However, we were successful in performing structural study of a newly discovered bacterial RNA repair complex consisting of three proteins named Pnkp1, Rnl and Hen1, which form a heterohexamer in vitro. Since the newly found RNA repair system possesses elements of both T4 and Pnkp–Hen1 RNA repair systems, it can be regarded as a hybrid RNA repair system. Therefore, the Pnkp1–Rnl–Hen1 heterohexamer is likely the functional unit of a new bacterial RNA repair system in vivo. Because the Pnkp1–Rnl–Hen1 RNA heterohexamer possesses two identical copies of each enzymatic activity, a total of eight active sites are present in the complex, same as in the RNA repair complex of the Pnkp–Hen1 heterotetramer.

To provide insight into the mechanism of RNA repair by the Pnkp1–Rnl–Hen1 heterohexamer, we soaked crystals with adenosine triphosphate (ATP) before data collection, which resulted in a crystal structure with cofactors occupying all active sites. Guided by the locations of these cofactors, and aided by the published structural homologues of Pnkp1 and Hen1 in complex with nucleic acids as well as the model of RNA in complex with the ligase module of Pnkp–Hen1, we manually docked short single-stranded RNAs into the four active sites located in the inner rim of one ring structure. The docking model shows that, while the reacting ends of single-stranded RNAs (not observed in Fig. 6a) are placed in the active site, the opposite ends point to a vacant space at the centre of the ring structure, indicating that a RNA substrate approaches each repair unit from this vacant space for RNA repair. The 5′ end of the damaged RNA would first enter the kinase site for phosphorylation and, at the same time, the 3′-end of the damaged RNA would go into the phosphatase site for dephosphorylation. Because of highly efficient 5′-phosphorylation carried out by the kinase domain of Pnkp1, the 5′ end would be the first to enter the ligase site, where it could be activated with 5′-adenylation by RNA ligase. On the other hand, after 3′-dephosphorylation carried out by the phosphatase domain of Pnkp1, the 3′ end could make a detour to the methyltransferase site of Hen1 for 2′-O-methylation before joining the 5′ end in the ligase site. With the presence of both processed ends in the ligase site, RNA ligation occurs, which results in repaired RNA with 2′-O-methylation. Among the four active sites located on the inner rim of the same ring structure, the kinase and phosphatase active sites are from one unit of the Pnkp1–Rnl–Hen1 heterotrimer, and the methyltransferase and ligase active sites are contributed from the other unit. Our structure revealed that the methyltransferase site is located between the phosphatase and ligase sites, providing the 3′ end of the damaged RNA maximal opportunity to be 2′-O-methylated after dephosphorylation but before ligation.

>MSAKNNTHHFPKLLILVGAPGSGKSTFARYFIRTEDNWVRVNRDDFRLMQFGDSLMSPFYEERITKMVEASVIALLKNRTNVIIDATNSSLRSLQDMVHTYTEYADISFKVFDLPVEELVKRCDKRCEQTGKFIPKSAIEKHVTQLQYTKEKFDFKPIPRALKETSLTYADQDTSLPKAVICDLDGTLSLLNGRDPYNASTADQDLLNTPVAMVLKMAKQQGYKVILLSGRENAYREPTERFLAKYQIDYDLLLMRDTNDYRKDNIIKKELFLEEIQGKYFVEFLLDDRNQVVDMWRRELALPCFQVNYGDF[2x];>[2x]MEDKTLIKKRIDWFCKNKINAFSPTISPAPKSVERNEIESLYEGILWFVLNGVKEIVIEKKYMGSYCDIYLHRRLEDTYLVSRNGYKINHLDQEQCLRALQGLHDRFSWDGVELRIIQSELMPWSILGKGLINNEFSAYYISHEIHAEYLVQSSLYEKLQKIQQEPAYLSFVADAKVLSAKELKDKYPMHIIRQYQSIRDFKFLDLPHYQQNIQLFKRQLDIFGKEAAPFFKPFNILKEVYTDGREHFVNDNLSFQQINDDDFLHYQFTDREDFEAKYPQIRAWVDQVNQSDEEGVVIKPRTAFLPGMPPAFKVRNNDYLTLVYGVDFEDRLQEQIAKRNIKGKLRCSINDWAINAKLLAIPYSELGEENYELKNLVLDRILGEEIENQLDSRL;>MILQIHSQNPHLLDLLNKNPHTDLGIYAKSLRNGQLIGNAVSAYQYDVVFQDTRYSYLPEESNQIDFQSYCSPLVILHICNEFFKELLQEKQTYWSQQIKWLERTRAEVDTYPCTIEVKNLYANSTWYSKGHFMMERYFKNIHITPIVGNNLSLRVEGKSVFEAMNLLSFIAVTTHITNTYGEYTYIDDHFAQKYARILTNIPQVPYFVFYLFIKRAIKSERQFAEIKPMFEAYFKEEGLDIDFQFTDTHGSRMDFIVKELGMEYPILDIGCGELKYYRRFMRRNYNYSHPYFATDTDKSVGDYAALLKERMEADNLYFFSDWTDYEYKNPVNIILTEVIEHNTPEAAEALVKHCLSLNFHKMIITTPNSLFNKYYFDEDPESLRHEDHHFEWTPQEFQDFIRHCVGDTSLEVTYCGIGDRINGETPTQAVVITRK[2x]> SNGGVIEELSCVRSNNYVQEPECRRNLVQCLLEKQGTPVVQGSLELERVMSSLLDMGFSNAHINELLSVRRGASLQQLLDIISEFILLGLNPEPVCVVLKKSPQLLKLPIMQMRKRSSYLQKLGLGEGKLKRVLYCCPEIFTMRQQDINDTVRLLKEKCLFTVQQVTKILHSCPSVLREDLGQLEYKFQYAYFRMGIKHPDIVKSEYLQYSLTKIKQRHIYLERLGRYQTPDKKGQTQIPNPLLKDILRVSEAEFLARTACTSVEEFQVFKKLLAREEEESESSTSDDKRASLDEDEDDDDEEDNDEDDNDEDDDDEDDDEAED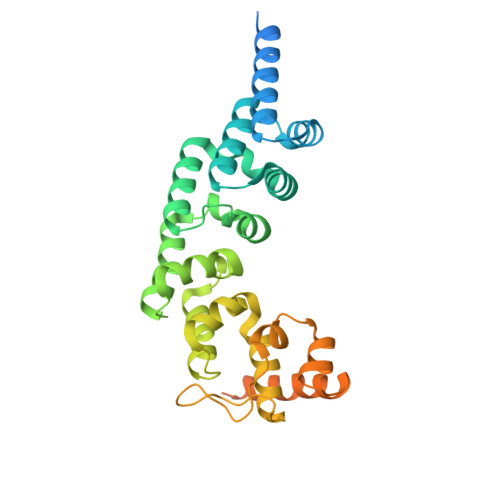NDEDEDDDEEE>CUUGCUGAAGCGCGCAC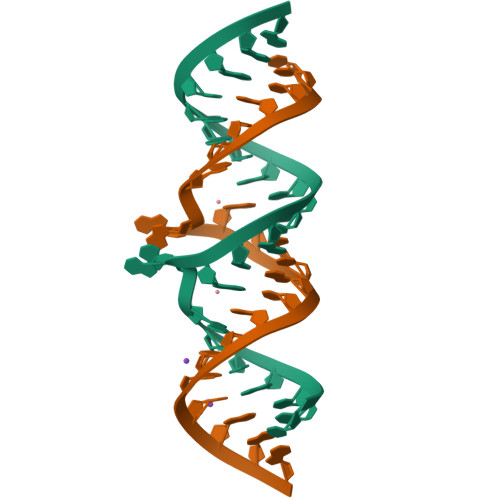GGCAAG[2x]>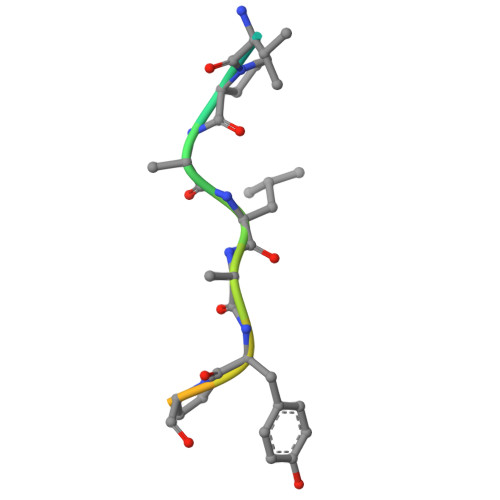 FTDVPALNYPATPPPH> MVRRSHVVAYYWSRYRMPTQMPKFDGPAPVAAPQSMNSTKTNEFIDPIDDKFPMSIRGPLVRPDVPEDQYVDSWYICTSMTHHMGDYRPWSASAPPNAFRFRPFNEFDAKGREYVQYMREFARFDPRKSRGNGQKGFPFRDAYLTKMNEANQKTPPPTLETIMDRAVREHHQHARILSPLEVQRDVGRLEPIPSYAGKINADRSVFPFQWKTEDWYEYEVAKVRNRRFVFENTEEDGIRGSEVTYKIVLEGFWDHHVMKLAEDVCMFLKDVGRQIVEEKLVAVRRLLQGGAVDPELLAAFNCARAGPFGGLDEYDKEEVANFLRSDLRRLEEQCLSVINRCNVPVPGATNIYDPHTSWPHVEKLEPWVRMAEFWTSSSDTSFTELEMSTAHYEFRKFFRVIICKLPFQSTEFEKRMYDIRHWLHRQTSCEFHTIYRRNVIHDSAVFPTEHDPATPTTHEHHRMFSFALDWQSAPVNRLSTDTVHEGESWDAVAQRLGCSVGELKDANAERETIEAGVVINVPVTATRRLTSFGATPLVLPLKTTSAKDGERIRTWEEAAAILDCTVEELQQCNGHAALTYQKKESEAGEFDSSETELVAPLSCWTSTSESEFSPVERVHANDTLVAIARRLQCSEEALRAVNDGITDVSGLDFVRVPPEARRPRRLVEPQLRPQAATDALLARTIAEEETFKLKSIPHLPQNAERFPHEYHTPTSRFPPTPSETPATQDWMAYTAKYLDKQFTISAEPAPVYNVNKLWPMQQIPGKVDQTPFEEDQTWLLHSIPVQQLEMHHHEKDL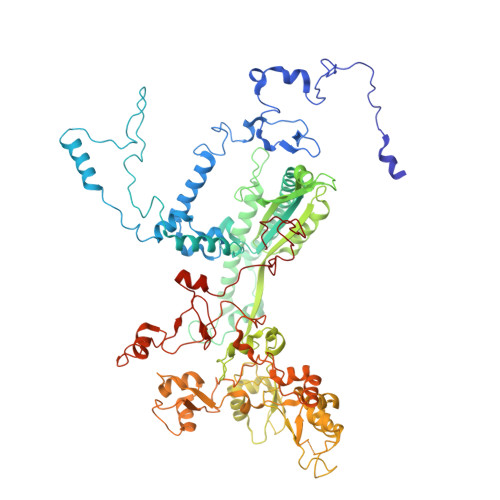QDLPFINHEQFPRSLEWNAP>MALSKVKLNDTLNKDQLLSSSKYTIQRSTGDSIDTPNYDVQKHINKLCGMLLITEDANHKFTGLIGMLYAMSRLGREDTIKILRDAGYHVKANGVDVTTHRQDINGKEMKFEVLTLASLTTEIQINIEIESRKSYKKMLKEMGEVAPEYRHDSPDCGMIILCIAALVITKLAAGDRSGLTAVIRRANNVLKNEMKRYKGLLPKDIANSFYEVFEKHPHFIDVFVHFGIAQSSTRGGSRVEGIFAGLFMNAYGAGQVMLRWGVLAKSVKNIMLGHASVQAEMEQVVEVYEYAQKLGGEAGFYHILNNPKASLLSLTQFPHFSSVVLGNAAGLGIMGEYRGTPRNQDLYDAAKAYAEQLKENGVINYSVLDL[20x]

HRSV belongs to the Mononegavirales order with the non-segmented negative-strand RNA genome fully coated by the viral nucleoprotein N. The resulting helical nucleocapsid (NC) shields the viral genetic material from recognition by the innate immune system while serving as template for replication and transcription by the viral RNA polymerase complex, thereby constituting a potential drug target. The helical HRSV nucleocapsid is a template for the viral RNA synthesis and a scaffold for the virion assembly. The helical NC, together with the RNA polymerase L, its phosphoprotein cofactor P and the transcription factor M2-1, form the HRSV RNA synthesis complex that constitues the minimal infectious unit of the virus. We explore the polymorphism of the nucleocapsid-like assemblies, report five structures of the full-length particles and two alternative arrangements formed by a C-terminally truncated nucleoprotein mutant, and demonstrate the functional importance of the identified longitudinal interfaces.

Since the structure of the helical HRSV NC demonstrates the involvement of the CTD-arm in the longitudinal contacts, we supposed that shortening of this arm may abrogate inter-turn interactions and thereby transform the non-canonical helix with asymmetric units composed of 16 N arranged in ~1.5 turns into a classical helix with one N per asymmetric unit. In spite of the truncation, the N1-370 mutant retained its interaction with P and therefore the corresponding N-RNA assemblies could be purified following the same protocol as the one used for the full-length (FL) construct and analysed by cryo-EM. The most glaring differences with the cryo-EM images of the full-length (FL) N-RNA were the appearance of two new types of coexisting filaments—the herringbone-like helices and a major population of unforeseen rigid stacks of rings. The rigid polymers coexisting with these helices are D10-symmetric and formed by alternating bottom-to-bottom and top-to-top packing of N10 rings. The ensuing 2.8 Å resolution cryo-EM map shows that the NTD-NTD stacked units are indistinguishable from the N10 double rings of FL N until the end of the α-helix 344–358 and the beginning of the CTD-arm. In the rings and helical assemblies of the FL N, the CTD-arm of the subunit Ni protrudes straight onto the top of the CTD of Ni+1. However, in the stacked rings of the N1-370 mutant, the truncated CTD-arm sharply pivots away and, instead of engaging into a lateral interaction, tucks into an identical site but on a CTD of the opposite ring in the stack. The pivoting of all CDT-arms tightly locks the adjacent rings together through their CTDs, such as to generate a polymer built of layers of inversely oriented N10 rings engaged both in NTD-NTD and CTD-CTD contacts; the latter are additionally stabilised by binding between CTD-arms of two opposing protomers, in particular through a Y365-Y365 stacking.> TMITNSRGSVDLQPSLTGVFPSGLIETKVSAAKITENYQFDSRIRLNSIGFIPNHSKKATIAANCSTFYVVKEDGTIVYTGTATSMFDNDTKETVYIADFSSVNEEGTYYLAVPGVGKSVNFKIAMNVYED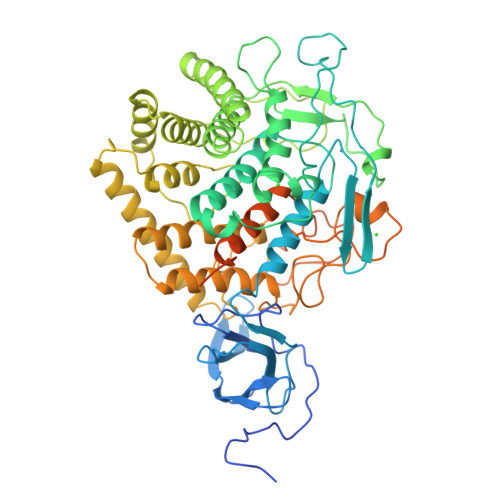AFKTAMLGMYLLRCGTSVSATYNGIHYSHGPCHTNDAYLDYINGQHTKKDSTKGWHDAGDYNKYVVNAGITVGSMFLAWEHFKDQLEPVALEIPEKNNSIPDFLDELKYEIDWILTMQYPDGSGRVAHKVSTRNFGGFIMPENEHDERFFVPWSSAATADFVAMTAMAARIFRPYDPQYAEKCINAAKVSYEFLKNNPANVFANQSGFSTGEYATVSDADDRLWAAAEMWETLGDEEYLRDFENRAAQFSKKIEADFDWDNVANLGMFTYLLSERPGKNPALVQSIKDSLLSTADSIVRTSQNHGYGRTLGTTYYWGCNGTVVRQTMILQVANKISPNNDYVNAALDAISHVFGRNYYNRSYVTGLGINPPMNPHDRRSGADGIWEPWPGYLVGGGWPGPKDWVDIQDSYQTNEIAINWNAALIYALAGFVNYNSPQNEVLYGDVNDDGKVNSTDLTLLKRYVLKAVSTLPSSKAEKNADVNRDGRVNSSDVTILSRYLIRVIEKLPI> ASSVNELENWSKWMQPIPDSIPLARISIPGTHDSGTFKLQNPIKQVWGMTQEYDFRYQMDHGARIFDIRGRLTDDNTIVLH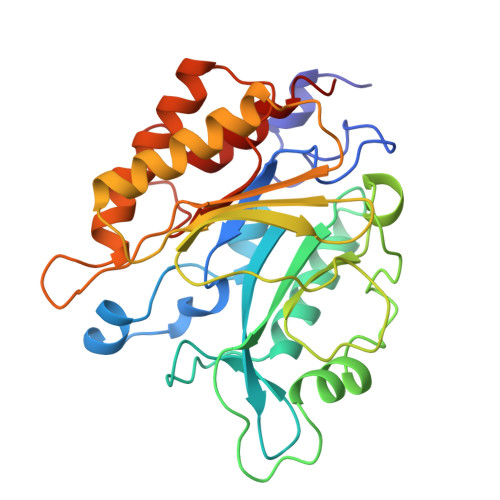HGPLYLYVTLHEFINEAKQFLKDNPSETIIMSLKKEYEDMKGAEDSFSSTFEKKYFVDPIFLKTEGNIKLGDARGKIVLLKRYSGSNEPGGYNNFYWPDNETFTTTVNQNANVTVQDKYKVSYDEKVKSIKDTMDETMNNSEDLNHLYINFTSLSSGGTAWNSPYYYASYINPEIANYIKQKNPARVGWVIQNYINEKWSPLLYQEVIRANKSLIKE1-DEAZA-ADENOSINE | C11 H14 N4 O4 | 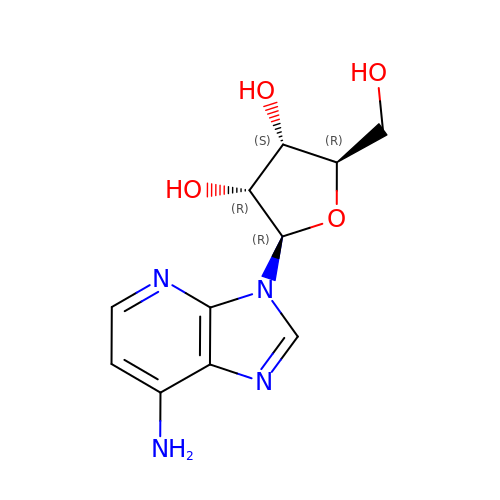NVUDDRWKCUAERS-PNHWDRBUSA-N>[4x]NNTLYFYNWTEYVPPGLLEQFTKETGIKVIYSTYESNETMYAKLKTYKDGAYDLVVPSTYYVDKMRKEGMIQKIDKSKLTNFSNLDPDMLNKPFDPNNDYSIPYIWGATAIGVNGDAVDPKSVTSWADLWKPEYKGS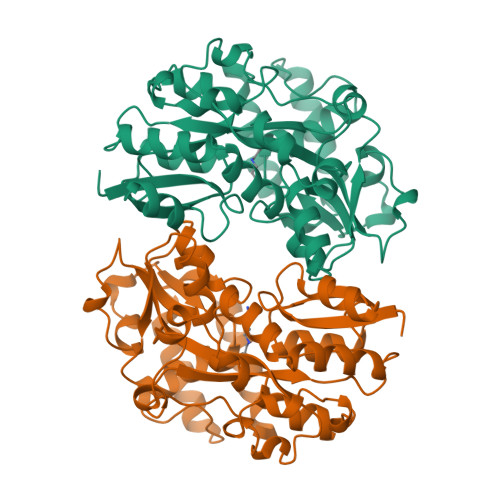LLLTDDAREVFQMALRKLGYSGNTTDPKEIEAAYNELKKLMPNVAAFNSDNPANPYMEGEVNLGMIWNGSAFVARQAGTPIDVVWPKEGGIFWMDSLAIPANAKNKEGALKLINFLLRPDVAKQVAETIGYPTPNLAARKLLSPEVANDKTLYPDAETIKNGEWQNDVGAASSIYEEYYQKLKAGR>GHMSTLLINQPQYAWLKELGLREENEGVYNGSWGGRGEVITTYCPANNEPIARVRQASVADYEETVKKAREAWKIWADIPAPKRGEIVRQIGDALREKIQVLGSLVSLEMGKILVEGVGEVQEYVDICDYAVGLSRMIGGPILPSERSGHALIEQWNPVGLVGIITAFNFPVAVYGWNNAIAMICGNVCLWKGAPTTSLISVAVTKIIAKVLEDNKLPGAICSLTCGGADIGTAMAKDERVNLLSFTGSTQVGKQVGLMVQERFGRSLLELGGNNAIIAFEDADLSLVVPSALFAAVGTAGQRCTTARRLFIHESIHDEVVNRLKKAYAQIRVGNPWDPNVL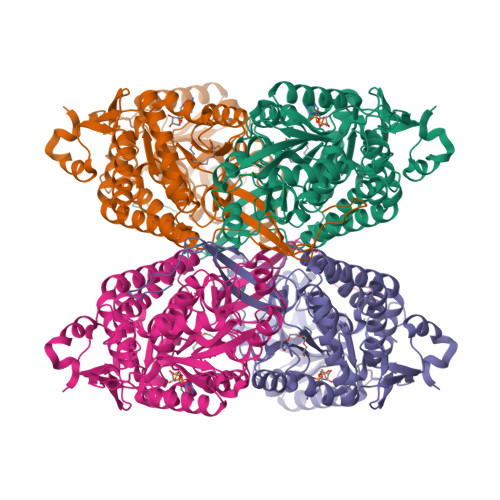YGPLHTKQAVSMFLGAVEEAKKEGGTVVYGGKVMDRPGNYVEPTIVTGLGHDASIAHTETFAPILYVFKFKNEEEVFAWNNEVKQGLSSSIFTKDLGRIFRWLGPKGSDCGIVNVNIPTSGAEIGGAFGGEKHTGGGRESGSDAWKQYMRRSTCTINYSKDLPLAQGIKFQ[8x]2-[(~{E},6~{R},10~{S})-6,10-bis(oxidanyl)undec-1-enyl]-4,6-bis(oxidanyl)benzoic acid | C18 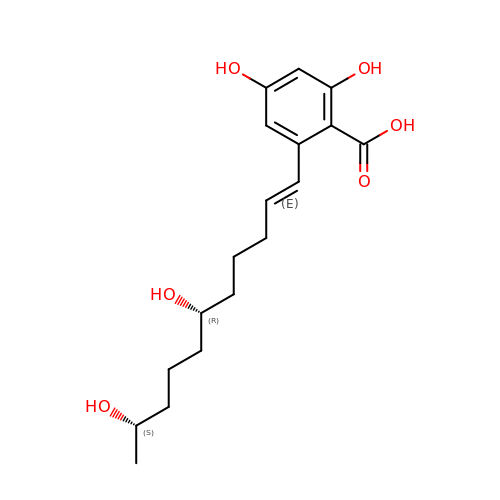H26 O6 | RSYOKTAWJDYBRR-QDKLYSGJSA-N>[4x]MGKLFGTFGVRGIANEKITPEFAMKIGMAFGTLLKREGRKKPLVVVGRDTRVSGEMLKEALISGLLSVGCDVIDVGIAPTPAVQWATKHFNADGGAVITASHNPPEYNGIKLLE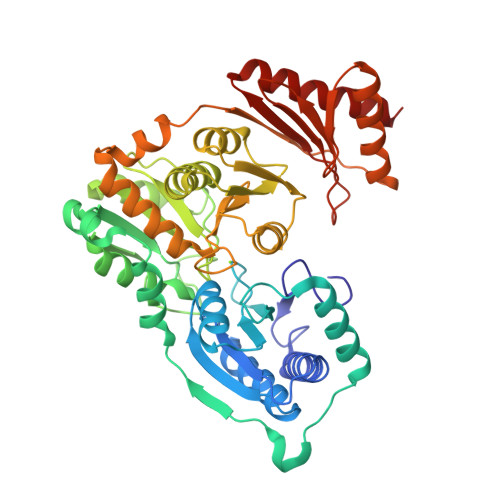PNGMGLKKEREAIVEELFFKEDFDRAKWYEIGEVRREDIIKPYIEAIKSKVDVEAIKKRKPFVVVDTSNGAGSLTLPYLLRELGCKVITVNAQPDGYFPARNPEPNEENLKEFMEIVKALGADFGVAQDGDADRAVFIDENGRFIQGDKTFALVADAVLKEKGGGLLVTTVATSNLLDDIAKKHGAKVMRTKVGDLIVARALYENNGTIGGEENGGVIFPEHVLGRDGAMTVAKVVEIFAKSGKKFSELIDELPKYYQIKTKRHVEGDRHAIVNKVAEMARERGYTVDTTDGAKIIFEDGWVLVRASGTEPIIRIFSEAKSKEKAQEYLNLGIELLEKALS> METNLFKLSLDDVETPKGSMLDLKISQSKIALPKNTVGGTILRSDLLANFLTEGNFRASVDLQRTHRIKGMIKMVATVGIPENTGIALACAMNSSIRGRASSDIYTICSQDCELWNPACTKAMTMSFNPNPCSDAWSLEFLKRTGFHCDIICVTGWTATPMQDVQVTIDWFISSQECVPRTY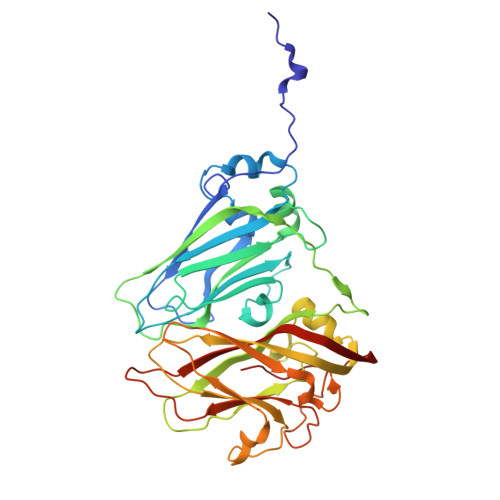CVLNPQNPFVLNRWMGKLTFPQGTSRSVKRMPLSIGGGAGAKSAILMNMPNAVLSMWRYFVGDLVFEVSKMTSPYIKCTVSFFIAFGNLADDTINFEAFPHKLVQFGEIQEKVVLKFSQEEFLTAWSTQVRPATTLLADGCPYLYAMVHDSSVSTIPGDFVIGVKLTIIENMCAYGLNPGISGSRLLG1-{2-[3,5-dicyclopropyl-4-(4-{[(quinoxaline-2-carbonyl)amino]methyl}-1H-1,2,3-triazol-1-yl)phenyl]acetamido}cyclohexane-1-carboxylic 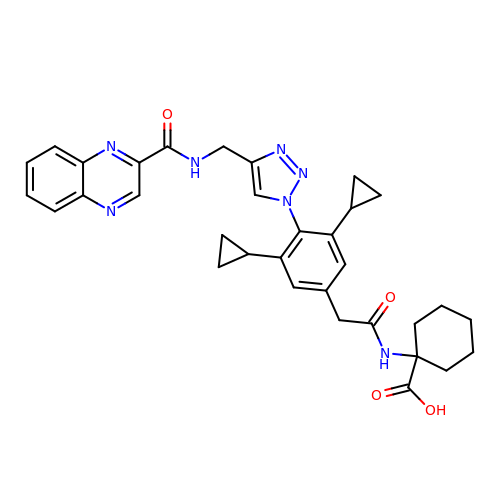acid | C33 H35 N7 O4 | BZXDUAKTLARJRN-UHFFFAOYSA-N>GSKDEKDHLIERLYREISGLKAQLENMKTESQRVVLQLKGHVSELEADLAEQQHLRQQAADDCEFLRAELDELRRQREDTEKAQ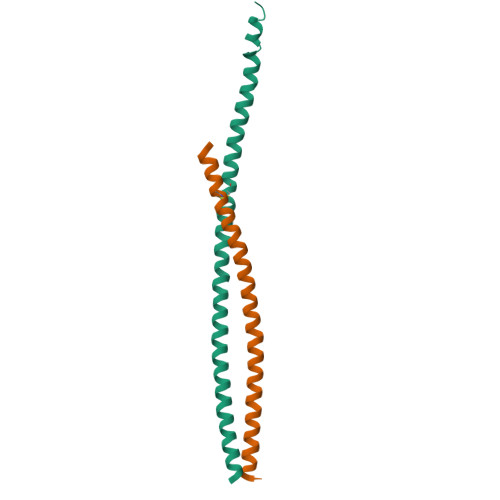RSLSEIERKAQANEQRYSKLKEKYSELVQN[4x]>[2x]GSHMSELEKAMVALIDVFHQYSGREGDKHKLKKSELKELINNELSHFLEEIKEQEVVDKVMETLDNDGDG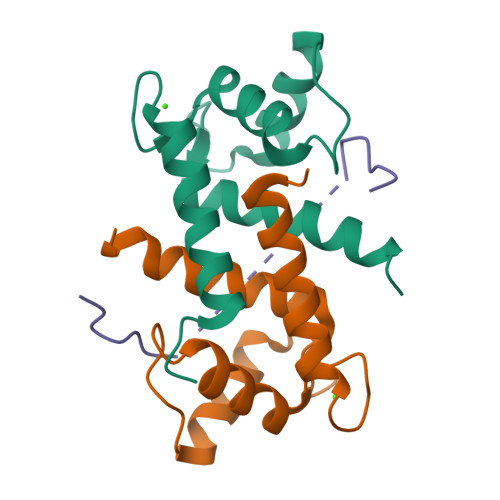ECDFQEFMAFVAMVTTACHEFFEHE;> GSQDLQLVKGAMAATYSALNSSKPTPQLKPIESSILAQRRVRKLPSTTL>[2x]HHHHHHGSVRIAMIGTGYVGLVSGACFSDFGHEVVCVDKDARKIELLHQNVMPIYEPGLDALVASNVKAGRLSFTTDLAEGVKDADAVFIAVGTPSRRGDGHADLSYVFAAAREIAENLTKPSVIVTKSTVPVGTGDEVERIIAEVAPNSGAKVVSNPEFLREGAAIEDFKRPDRVVVGTEDEFARQVM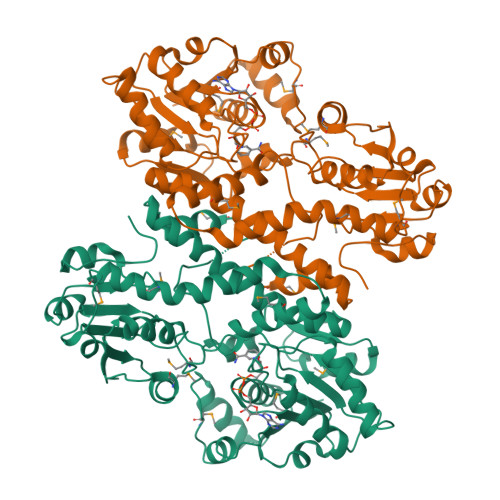REIYRPLSLNQSAPVLFTGRRTSELIKYAANAFLAVKITFINEIADLCEQVGADVQEVSRGIGMDNRIGGKFLHAGPGYGGSCFPKDTLALMKTAADNETPLRIVEATVQVNDARKRAMGRKVIKAMGGDVRGKTVGILGLTFKPNTDDMRDAPSLSIIAALQDAGATVKAYDPEGVEQASKMLTDVEFVENPYAAADGADALVIVTEWDAFRALDLTRIKNSLKSPVLVDLRNIYPPAELERAGLQYTGVGKPSRD BAZ2A is an epigenetic regulator affecting transcription of ribosomal RNA. It is overexpressed in aggressive and recurrent prostate cancer, promoting cellular migration. BAZ2A, however, features a shallow pocket, making it one of the least druggable bromodomains. Here, we describe a structure-based fragment-growing campaign for the identification of ligands of the BAZ2A bromodomain.

The IC50 values for the isoamyl derivative 79 and the bicyclic tetrahydroisoindol-4-one analogs 80 and 81 are 3 times lower than that measured for 47. Crystallographic structures of compounds 77–80 show almost superimposable poses for the five inhibitors. Extensive contacts with Leu1826 and Val1827 are formed by the bulkier substituents of compounds 78–79.

> SMHSDLTFCEIILMEMESHDAAWPFLEPVNPRLVSGYRRIIKNPMDFSTMRHRLSRGGYTSSEEFAADALLVFDNCQTFNEDDSEVGKAGHIMRRFFESRWEEFYQ> MELKHSISDYTEAEFLE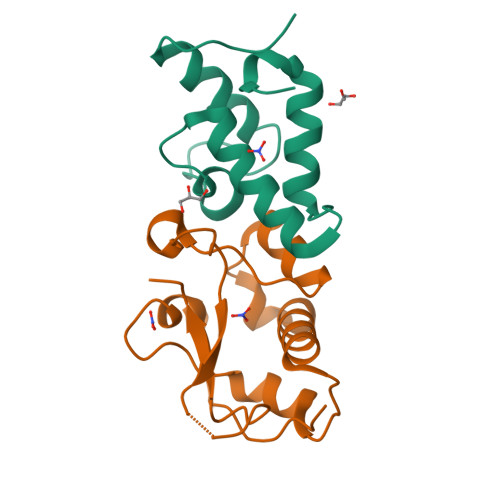FVKKIARAEGATECDDNKLVREFERLTEHPDGSDLIYYPRDDREDSPEGIVKEIKEWRAANGKSGFKQG;> MESKRNKPGKATGKGKPVGDKWLDDAGKDSGAPIPDRIADKLRDKEFKSFDDFRKAVWEEVSKDPELSKNLNPSNKSSVSKGYSPFTPKNQQVGCRKVYELHHDKPISQGGEVYDMDNIRVTTPKRHIDIHRGK>[4x]GSHMTGGSVHSSPAIGQDGTIYVGSNDHYLYAINPNGKLKWKFETGGSVHSSPAIGQDGTIYVGSNDHYLYAINPNGKLKWKFETGGSVHSSPAIGQDGTIYVGSNDH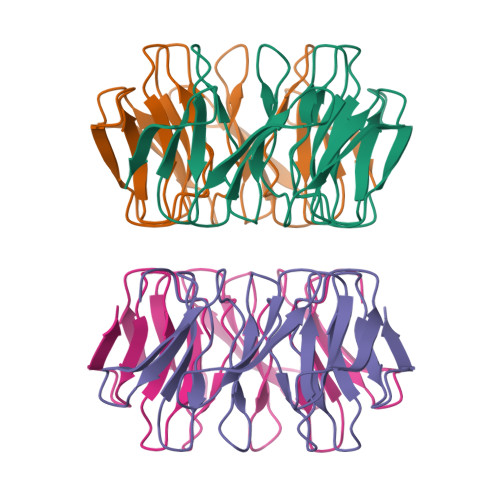YLYAINPNGKLKWKFETGGSVHSSPAIGQDGTIYVGSNDHYLYAINPNGKLKWKFE> DKYETNVSYKKLNQLAPYFKGFDGSFVLYNEREQAYSIYNEPESKQRYSPNSTYKIYLALMAFDQNLLSLNHTEQQWDKHQYPFKEWNQDQNLNSSMKYSVNWYYENLNKHLRQDEVKSYLDLIEYGNEEISGNENYWNESSLKISAIEQVNLLKNMKQHNMHFDNKAIEKVENSMTLKQKDTYKYVGKTGTGIVNHKEANGWFVGYVETKDNTYYFATHLKGEDNANGEKAQQISERILKEMELI;> G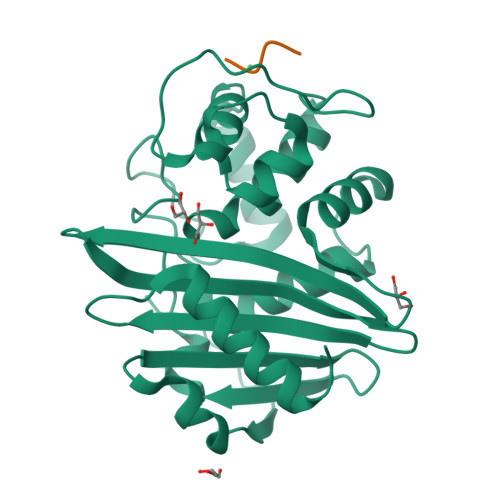HMS>[2x]HTSPLLAPVRQIHAFGDAYSDNGESQRLTREMLAKGIAGAQALPGEVYWQGRWSNGPTAVEVLARQLGAQLADHAVGGAKSGADNYYGWMSAYRHTGLAGQVDAYLATLDGKPVDGQALHFIFVSANDFFE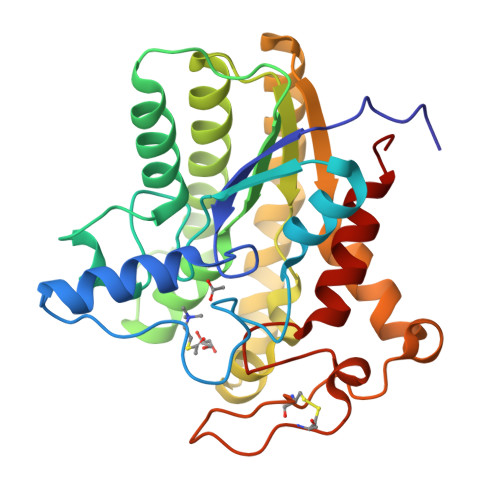HEDFAGEQPLEQLAGSSVANIRAAVQRLGEAGARRFLVVSSTDLSVVPAVVAGNRVERAQRYLQAVNASLPIQLAALRKTRGLELSWFDHLTFSRHLRRNPARYGLVELDAPCQPTQPSVRPACANPDQYYFWDEWHPTRRVHQLAGEAMAARYAR N-[2-(5,6-dimethyl-1H-benzimidazol-2-yl)ethyl]-4-(4H-1,2,4-triazol-4-yl)benzamide | C20 H20 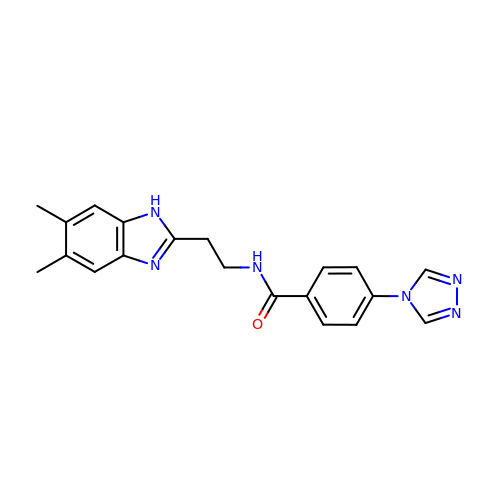N6 O | QNOXZLGNUKPKFJ-UHFFFAOYSA-N> MGSSHHHHHHSSGTIEGRMIRLTDNRPIGFIDSGVGGLTVVKEALKQLPNENILFVGDTARCPYGPRPAEQVIQYTWEMT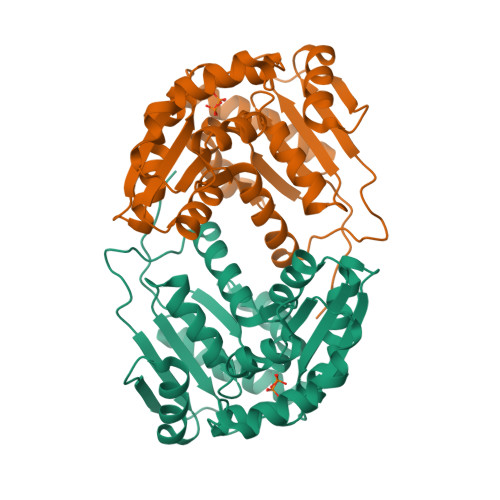DYLVEQGIKMLVIACNTATAVALEEIKAALSIPVIGVILPGTRAAVKKTQNKQVGIIGTIGTVKSQAYEKALKEKVPELTVTSLACPKFVSVVESNEYHSSVAKKIVAETLAPLTTKKIDTLILGCTHYPLLRPIIQNVMGENVQLIDSGAETVGEVSMLLDYFNLSNSPQNGRTLCQFYTTGSAKLFEEIAEDWLGIGHLNVEHIELGGK> GSNGVSEAELLTKTLPDILTFNLDIVIIGINPGLMAAYKGHHYPGPGNHFWKCLFMSGLSEVQLNHMDDHTLPGKYGIGFTNMVERTTPGSKDLSSKEFREGGRILVQKLQKYQPRIAVFNGKC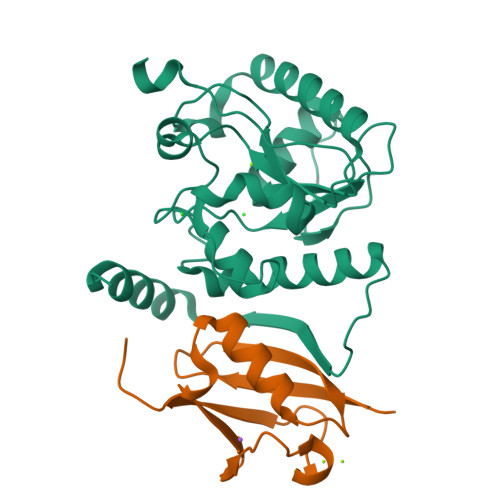IYEIFSKEVFGVKVKNLEFGLQPHKIPDTETLCYVMPSSSARCAQFPRAQDKVHYYIKLKDLRDQLKGIERNMDVQEVQYTFDLQLAQEDAKKMAVKEEKYDPGYE;> MSDQEAKPSTEDLGDKKEGEYIKLKVIGQDSSEIHFKVKMTTHLKKLKESYCQRQGVPMNSLRFLFEGQRIADNHTPKELGMEEEDVIEVYQEQTGG> SNAMPYTWKFLGISKQLSLENGIAKLNQLLNLEVDLDIQTIRVPSDPDGGTAADEYIRYEMRLDISNLDEGTYSKFIFLGNSKMEVPMFLCYCGTDNRNEVVLQWLKAEYGVIMWPIKFEQKTMIKLADASIVHVTKENIEQITWFSSKLYFEPETQDKNLRQFSIEIPRESCEGLALGYGNTMHPYNDAIVPYIYNETGMAVERLPLTSVILAGHTK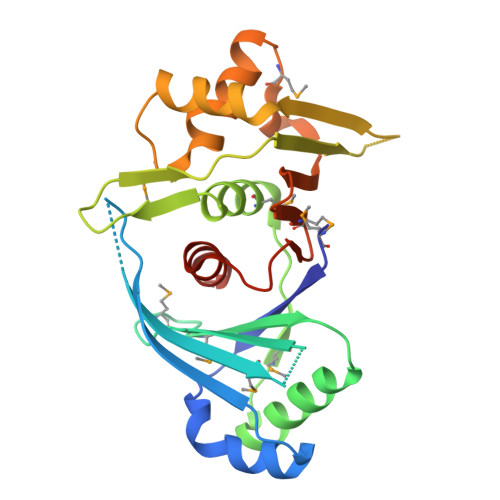IMRESIVTSTRSLRNRVLAVVLQSIQFTSE> PKYTDKEVQQISGNLNLNIVPLFEKTLSASDAGRIGRLVLPKACAEAY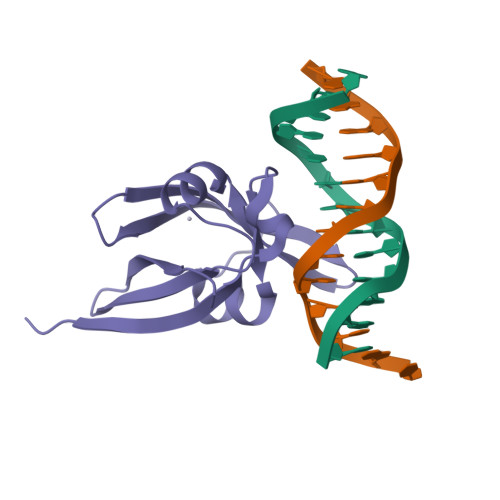FPPISQSEGIPLKIQDVRGREWTFQFRYWPNNNSRMYVLEGVTPCIQSMMLQAGDTVTFSRVDPGGKLIMGSRKAANAGD4,5,6-TRIHYDROXY-7-HYDROXYMETHYL-4,5,6,7-TETRAHYDRO-1H-[1,2,3]TRIAZOLO[1,5-A]PYRIDIN-8-YLIUM 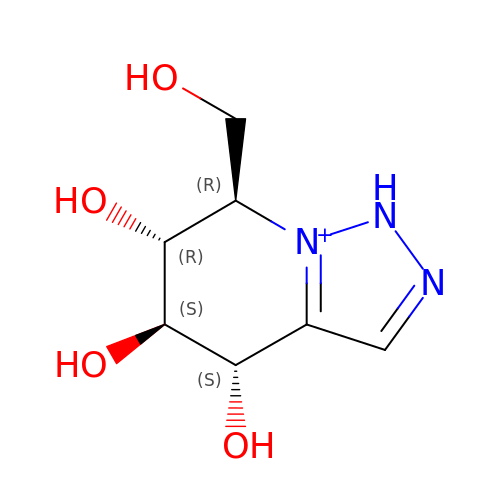| C7 H12 N3 O4 | QTNWFPNNMUCBLD-XZBKPIIZSA-O>MSEQLVTPENVTTKDGKINLLDLNRQQMREFFKDLGEKPFRADQVMKWMYHYCCDNFDEMTDINKVLRGKLKEVAEIRAPEVVEEQRSSDGTIKWAIAVGDQRVETVYIPEDDRATLAVSSQVGCALECKFCSTAQQGFNRNLRVSEIIGQVWRAAKIVGAAKVTGQRPITNVVMMGMGEPLLNLNNVVPAMEIMLDDFGFGLSKRRVTLSTSGVVPALDKLGDMIDVALAISLHAPNDEIRDEIVPINKKYNIET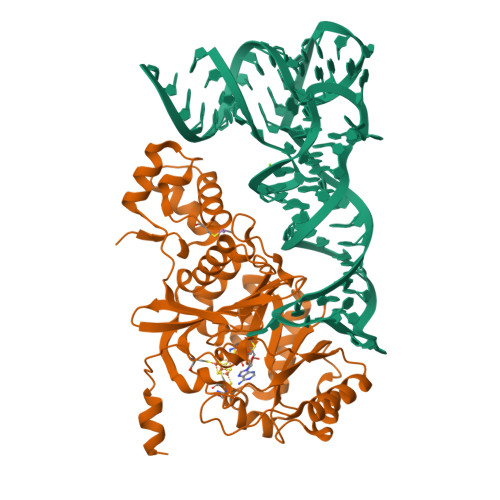FLAAVRRYLEKSNANQGRVTIEYVMLDHVNDGTEHAHQLAELLKDTPCKINLIPWNPFPGAPYGRSSNSRIDRFSKVLMSYGFTTIVRKTRGDDIDAACGQLAGDVIDRTKRTLRKRMQGEAIDIKAVGNSSSVDKLAAALEHHHHHH[2x]>[2x]MHHHHHHSSGSSSTGSSAAAVASKQRRRSSYAFNNGNGATNLNKSGGKKFILELIETVYEEILDLEANLRNGQQTDSTAMWEALHIDDSSYDVNPFISMLSFDKGIKIMPRIFNFLDKQQKLKILQKIFNELSHLQIIILSSYKTTPKPTLTQLKKVDLFQMIILKIIVSFLSNNSNFIEIMGLLLQLIRNNNVSFLTTSKIGLNLITILISRAALIKQDS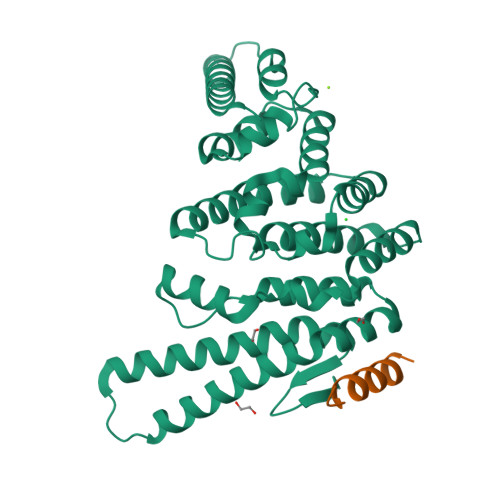SRSNILSSPEISTWNEIYDKLFTSLESKIQLIFPPREYNDHIMRLQNDKFMDEAYIWAFLASLAASGKLNHQRIIIDEVRDEIFATINEAETLQKKEKELSVLPQRSQELDTELKSIIYNKEKLYQDLNLFLNVMGLVYRDGEISELK;>[2x]TAHSNSQALLDLLKKPT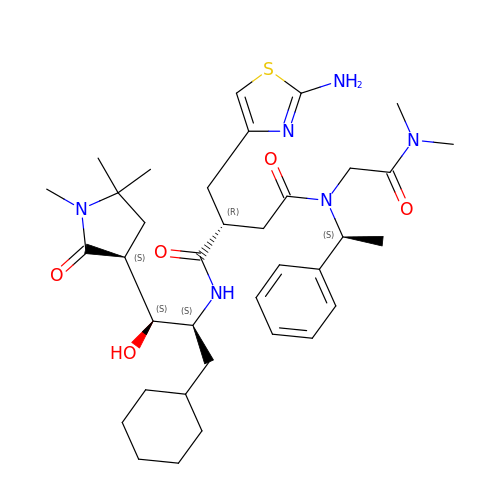(2S)-2-[(2-amino-1,3-thiazol-4-yl)methyl]-N~1~-{(1S,2S)-1-(cyclohexylmethyl)-2-hydroxy-2-[(3R)-1,5,5-trimethyl-2-oxopyrrolidin-3-yl]ethyl}-N~4~-[2-(dimethylamino)-2-oxoethyl]-N~4~-[(1S)-1-phenylethyl]butanediamide | C36 H54 N6 O5 S | IFJSAOFSWZWPQF-SQMKVVGDSA-N> QTEDYCLASNKVGRC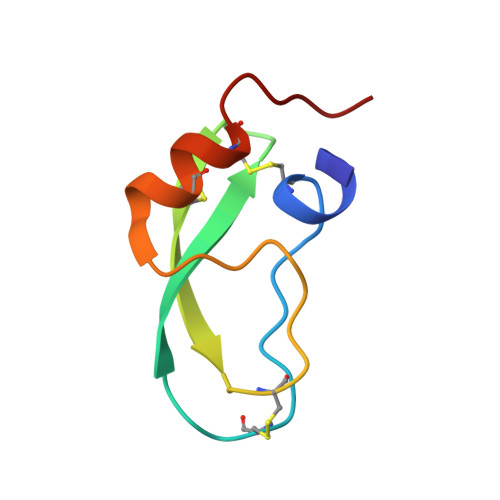RGSFPRWYYDPTEQICKSFVYGGCLGNKNNYLREEECILACRGVQGP>[2x]MGSEMSEMSVVDYVVTSFNSTSQMSHELLFSVKKRWFVKPFEHSRRYG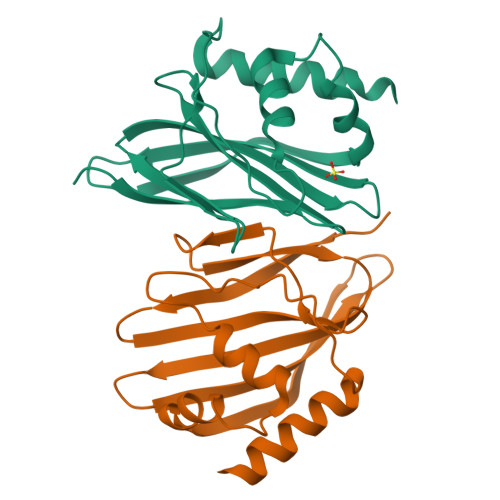LLAYMLLPGNYIKFGLYVLKNQDYARFEIAWVHVDKDGKIEERTVYSIETYWHIFIDIENDLNCPYVLAKFIEMRPEFEKTAWVEESNYSIAEDDIQMVESIKRYLERKIASD(1~{S},2~{S})-1-[(4-methylphenyl)methyl]-2-phenyl-cyclopropane-1-carboxylic acid 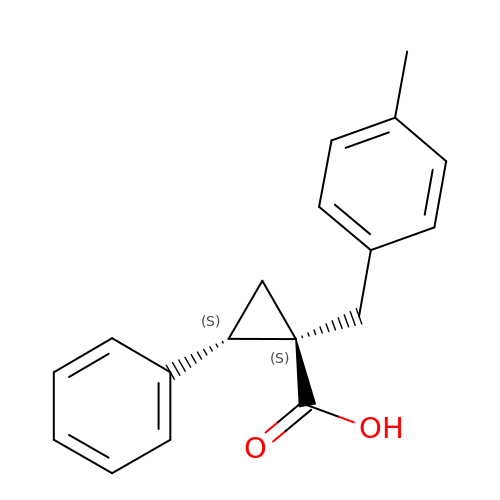| C18 H18 O2 | AKNVQFLVLPRHIR-FUHWJXTLSA-N>GSHMGGVEVLEVKTGVDSITEVECFLTPEMGDPDEHLRGFSKSISISDTFESDSPNRDMLPCYSVARIPLPNLNEDLTCGNILMWEAVTLKTEVIGVTSLMNVHSNGQATHDNGAGKPVQGTSFHFFSVGGEALELQGVLFNYRTKYPDGTIFPKNATVQSQVMNTEHKAYLDKNKAYPVECWVPDPTRNENTRYFGTLTGGENVMPVLHITNTATTVLLDEFGVGPLCKGDNLYLSAVDVCGMFTNRSGSQQWRGLSRYFKV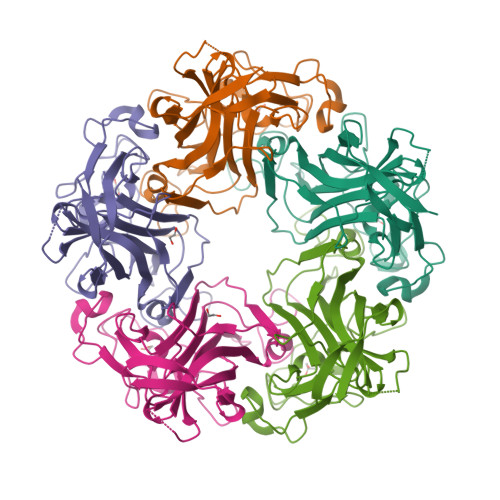QLRKRRVKN[5x]>[2x]MKIVLVLYDAGKHAADEEKLYGCTENKLGIANWLKDQGH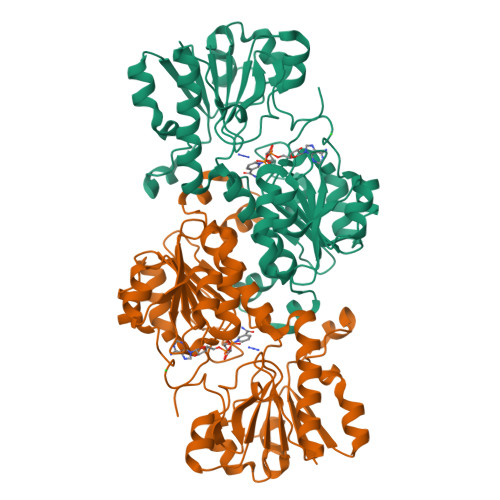ELITTSDKEGGNSVLDQHIPDADIIITTPFHPAYITKERIDKAKKLKLVVVAGVGSDHIDLDYINQTGKKISVLEVTGSNVVSGAEHVLMTMLVLVRNFVPAHEQIINHDWEVAAIAKDAYDIEGKTIATIGAGRIGYRVLERLVPFNPKELLYYDYQALPKDAEEKVGARRVENIEELVAQADIVTINAPLHAGTKGLINKELLSKFKKGAWLVNTARGAICVAEDVAAALESGQLRGYGGDVWFPQPAPKDHPWRDMRNKYGAGNAMTPHYSGTTLDAQTRYAEGTKNILESFFTGKFDYRPQDIILLNGEYITKAYGKHDKK>[2x]MSKNYHIAVLPGDGIGPEVMAQALKVMDAVRSRFDMRITTSHYDVGGIAIDNHGHPLPKATVEGCEQADAILFGSVGGPKWENLPPESQPERGALLPLRKHFKLFSNLRPAKLYQGLEAFCPLRADIAANGFDILCVRE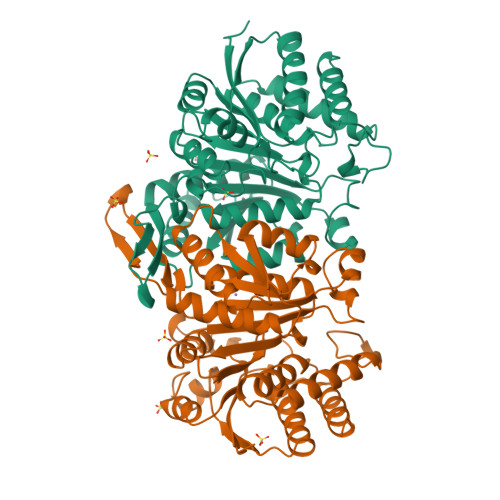LTGGIYFGQPKGREGSGQYEKAFDTEVYHRFEIERIARIAFESARKRRRKVTSIDKANVLQSSILWREIVNDVAKTYPDVELAHMYIDNATMQLIKDPSQFDVLLCSNLFGDILSDECAMITGSMGMLPSASLNEQGFGLYEPAGGSAPDIAGKNIANPIAQILSLALLLRYSLDANDAATAIEQAINRALEEGVRTGDLARGAAAVSTDEMGDIIARYVAEGV> THVDLGLASANVDFAFSLYKQLVLKAPDKNVIFSPLSISTALAFLSLGAHNTTLTEILKGLKFNLTETSEAEIHQSFQHLLRTLNQSSDELQLSMGNAMFVKEQLSLLDRFTEDAKRLYGSEAFATDFQDSAAAKKLINDYVKNGTRGKITDLIKDLDSQTMMVLVNYIFFKAKWEMPFDPQDTHQSRFYLSKKKWVMVPMMSLHHLTIPYFRDEELSCTVVELKYTGNASALFILPDQDKMEEVEAMLLPETLKRWRDSLEFREIGELYLPKFSISRDYNLNDILLQLGIEEAFTSKADLSGITGARNLAVSQVVHKAVLDVFEEGREASAATAVKITLL;> VETRTIVRFNRPFLMIIVPTDTQNIFFM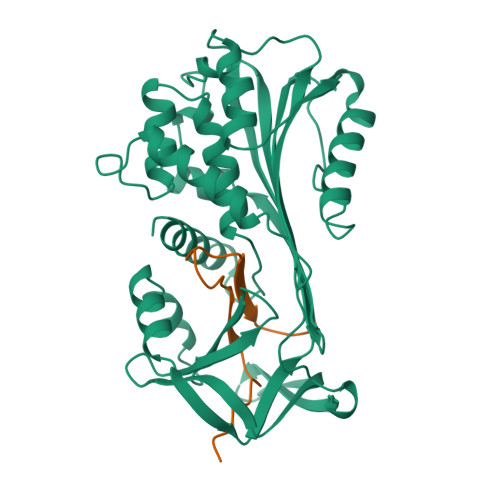SKVTNPKQA> XTVINLFAPGK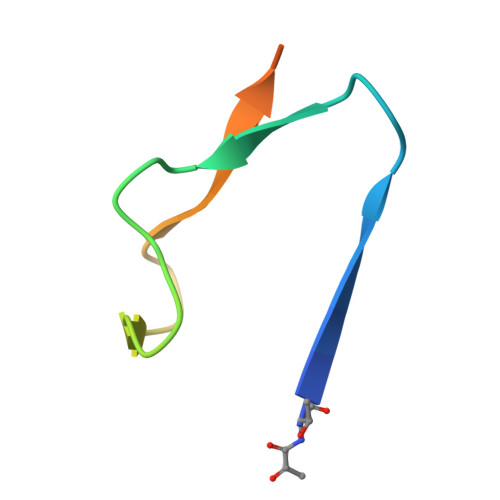VNLVEQLESLSVTKIGQPLAVSTGHHHHHHG6-aminohexan-1-ol | C6 H15 N O | 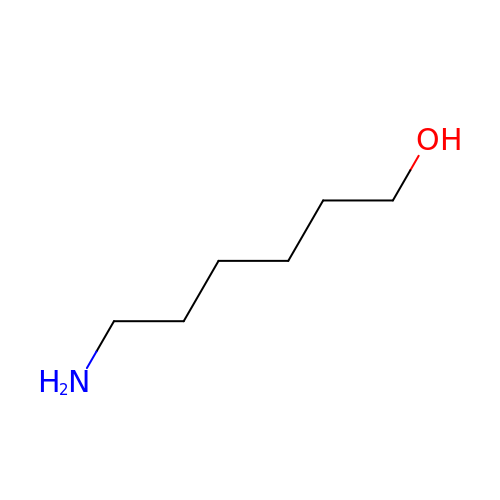SUTWPJHCRAITLU-UHFFFAOYSA-N> GGUAAGGUCAUGUUCGUGGUUGAAAGUCCAAGCCAGCUACGGG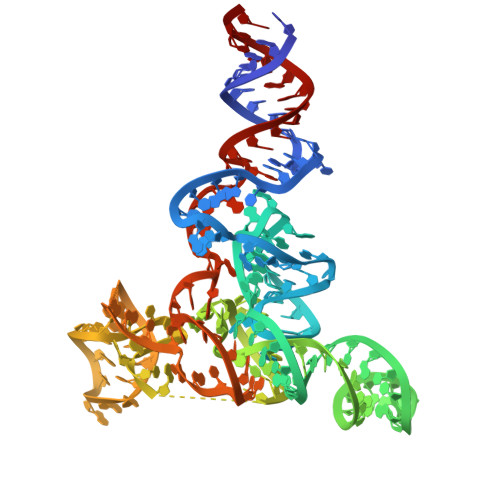CAAAGGGAUCCACGUAAGCUGCUGCGGAGACGGCAGUGAUCAUGGCGUAGCUUAGAAGUAAGUCCUCCGGGAAACUCGGGUUAAGGCAAGUGUGGGGUCAAAAACCAGGUCGAGUGGCCUUG> KIFKPEELRQALMPT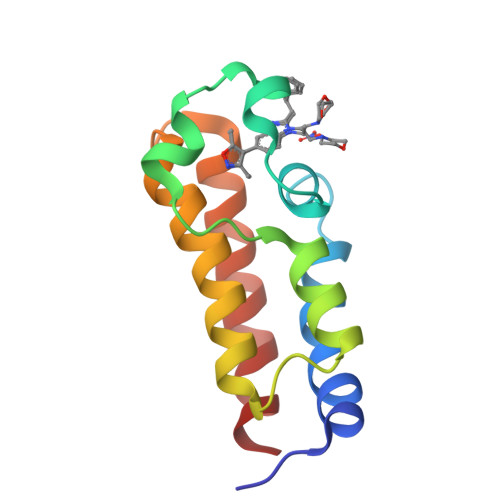LEALYRQDPESLPFRQPVDPQLLGIPDYFDIVKNPMDLSTIKRKLDTGQYQEPWQYVDDVWLMFNNAWLYNRKTSRVYKFCSKLAEVFEQEIDPVMQS> YSIEADKKFKYSVKLSDYPTLQDAASAAVDGLLIDRDYNFYGGETVDFG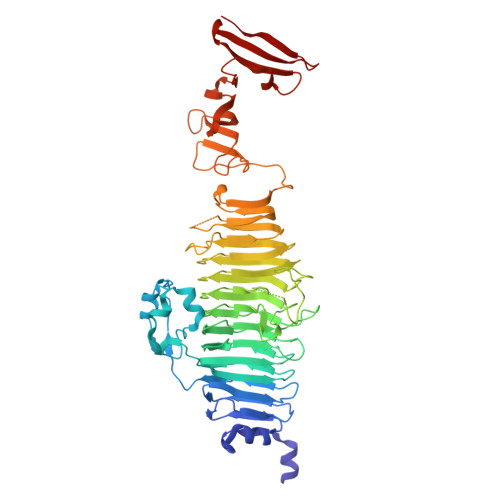GKVLTIECKAKFIGDGNLIFTKLGKGSRIAGVFMESTTTPWVIKPWTDDNQWLTDAAAVVATLKQSKTDGYQPTVSDYVKFPGIETLLPPNAKGQNITSTLEIRECIGVEVHRASGLMAGFLFRGCHFCKMVDANNPSGGKDGIITFENLSGDWGKGNYVIGGRTSYGSVSSVQFLRNNGGFERDGGVIGFTSYRAGESGVKTWQGTVGSTTSRNYNLQFRDSVVIYPVWDGFDLGADTDMNPELDRPGDYPITQYPLHQLPLNHLIDNLLVRGALGVGFGMDGKGMYVSNITVEDCAGSGAYLLTHESVFTNIAIIDTNTKDFQANQIYISGACRVNGLRLIGIRSTDGQGLTIDAPNSTVSGITGMVDPSRINVANLAEEGLGNIRANSFGYDSAAIKLRIHKLSKTLDSGALYSHINGGAGSGSAYTQLTAISGSTPDAVSLKVNHKDCRGAEIPFVPDIASDDFIKDSSCFLPYWENNSTSLKALVKKPNGELVRLTLATL In this work, we exhaustively probe the ability of all 36 immobile HJ sequences to form DNA crystals in two different designed systems. Three separate self-assembling DNA crystal systems are described in this report: the “4 × 5” and “4 × 6” designs (collectively referred to as the 4 × N systems), and a third construct with a “scrambled” sequence variant of the 4 × 6 lattices. Self-assembly was mediated by three constituent oligonucleotides: (S1) containing four sequence repeats of either 5 or 6 bases; (S2) composed of 21 bases containing complementary regions to both (S1); and (S3) which forms the second junction crossover. The HJ serves as the fundamental component at the core of each unit, and the ultimate assembly of the full lattice is facilitated by the complementary 2-base sticky ends that tail each duplex.

To investigate this possibility, we designed “scrambled” sequences with targeted base substitutions, while maintaining GC content, along each “stem”. Contrary to the buffer preference observed with the native P32 crystals, the scrambled systems exhibited an exclusive preference towards low salt buffers, much like the native R3 crystals. Remarkably, only J1 and J2 retained the P32 symmetry, with all others yielding an R3 lattice. There appeared to be only a marginal difference in the average cell lengths in the R3 scramble crystals (a = b = 113.04 c = 51.10) relative to the native 4 × 6 sequences: the a, b axis trended ~2 Å shorter and c ~1.3 Å longer, whereas in the J1 and J2 cases, the crystals were in good agreement with the original 4 × 6 motif. The average angles of the R3 and P32 crystals were 61.00° (σ = 1.21) and 58.05° (σ = 1.39), respectively. Another major observation is the importance of stem region sequences outside the HJ, given that this sequence can control crystal symmetry and lattice architecture, and improve resolution in non-obvious ways. However, in the majority of the crystal structures reported here, the cacodylate anion indeed fits best into the electron density map of our X-ray structures, due to the presence of sodium cacodylate in the crystallization solution.

> GAACGACACTGA;> CGGGGACTC;> TCACCG;> TCGAGTCCGTGTCGT>[2x]GAMDMKITLFSSKPYWVKWFNELNKFSYEINYVTSACDIKSVN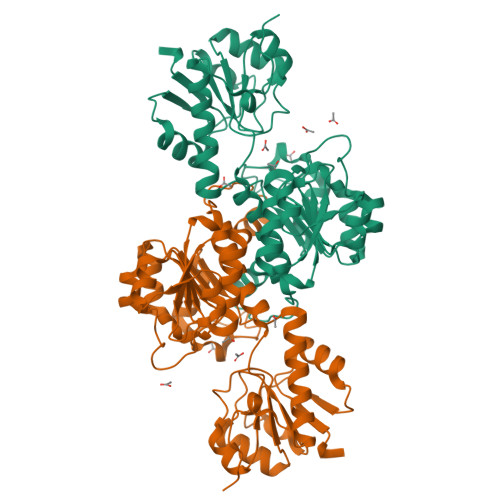EAKGSEAVCCFVNDDLSKEVIETLHSNGTKVILMRCAGFNKVDLDTANKLGIPVLRVPAYSPNAVSEYALSLIMALNRKTHKAHDRVRDANFEINGMEGFNMVSKVYGIVGTGNIGEQLCRVLKLGFGAKVIAYDIIENKAVTDIGIEYVKTLDEIWKQCDVISLHTPLNSQTKYMVNSESIEKMRDGVMIINVSRGALVNASDAIVGLKSGKISSLGMDVYENETDYFYQDHNGSIIKDDNLSLLISYPNVMITSHQAWYTKEAISCICGTSLQNFVDFRSNQIKKSNLVNNPISSQPTQ>[2x]MLLEAIFHEAKGSYAYPISETQLRVRLRAKKGDVVRCEVLYADRYASPEEELAHALAGKAGSDERFDYFEALLECSTKRVKYVFLLTGPQGEAVYFGETGFSAERSKAGVFQYAYIHRSEVFTTPEWAKEAVIYQIFPERFANGDPSNDPPGTEQWAKDARPRHDSFYGGDLKGVIDRLPYLEELGVTALYFTPIFASPSHHKYDTADYLAIDPQFGDLPTFRRLVDEAHRRGIKIILDAVFNHAGDQFFAFRDVLQKGEQSRYKDWFFIEDFPVSKTSRTNYETFAVQVPAMPKLRTENPEVKEYLFDVARFWMEQGIDGWRLNVANEVDHAFWREFRRLVKSLNPDALIVGEIWHDASGWLMGDQFDSVMNYLFRESVIRFFATGEIHAERFDAELTRARML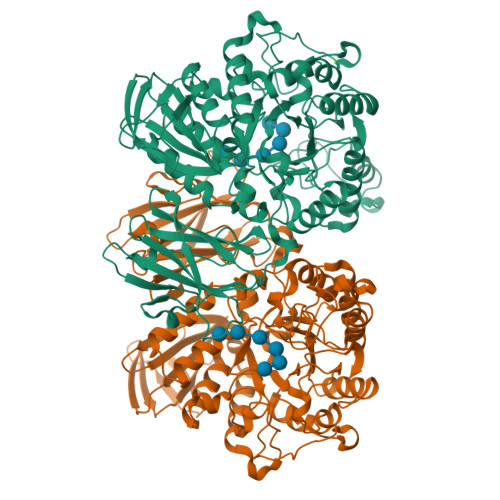YPEQAAQGLWNLLDSHDTERFLTSCGGNEAKFRLAVLFQMTYLGTPLIYYGDEIGMAGATDPDCRRPMIWEEKEQNRGLFEFYKELIRLRHRLASLTRGNVRSWHADKQANLYAFVRTVQDQHVGVVLNNRGEKQTVLLQVPESGGKTWLDCLTGEEVHGKQGQLKLTLRPYQGMILWNGR> MDPDQYSIEADKKFKYSVKLSDYPTLQDAASAAVDGLLIDRDYNFYGGETVDFGGKVLTIECKAKFIGDGNLIFTKLGKGSRIAGVFMESTTTPWVIKPWTDDNQWLTDAAAVVATLKQSKTDGYQPTVSDYVKFPGIETLLPPNAKGQNITSTLEIRECIGVEVHRASGLMAGFLFRGCHFCKMVDANNPSGGKDGIITFENLSGDWGKGNYVIGGRTSYGSVSSAQFLRNNGGFERDGGLIGFTSYRAGESGVKTWQGTVGSTTSRNYNLQFRDSVVIYPVWDGFDLGADTDMNPELDRPGDYPITQYPLHQLPLNHLIDNLLVRGALGVGFGMDGKGMYVSNITVEDCAGSGAYLLTHESVFTNIAIIDTNTKDFQANQIYISGACRVNGLRLIGIRSTDGQSLTIDAPNSTVSGITGMVDPSRINVANLAEEGLGNIRANSFGYDSAAIKLRIHKLSKTLDSGALYSHINGGAGSGSAYTQLTAISGSTPDAVSLKVNHKDCRGAEIPFVPDIASDDFIKDSSCFLPYWENN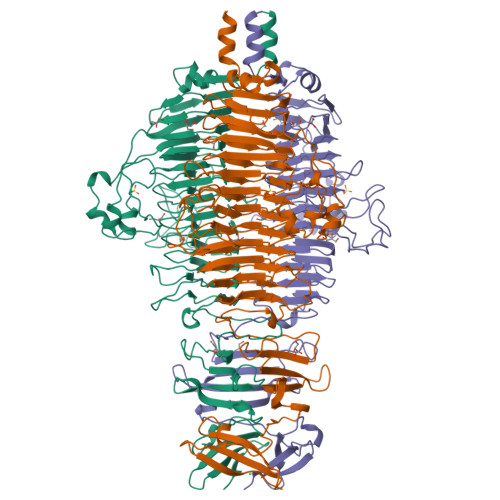STSLKALVKKPNGELVRLTLATL>GSDSHSKQLEINVKSDKVPQKVKDLAQQQFAGYAKALDKQSNAKTGKYELGEAFKIYKFNGEEDNSYYYPVIKDGKIVYTLTLSPKNKDDLNKSKEDMNYSVKISNFIAKDLDQIKDKNSNITVLTDEKGFYFEEDGKVRLVKATPLANNIKEKESAKTVSPQLKQELKTTVTPTKVEENEAIQEDQVQYENTLKNFKIREQQFDNSWCAGFSMAALLNATKNTDTYNAHDIMRTLYPEVSEQDLPNCATFPNQMIEYGKSQGRDIHYQEGVPSYNQVDQ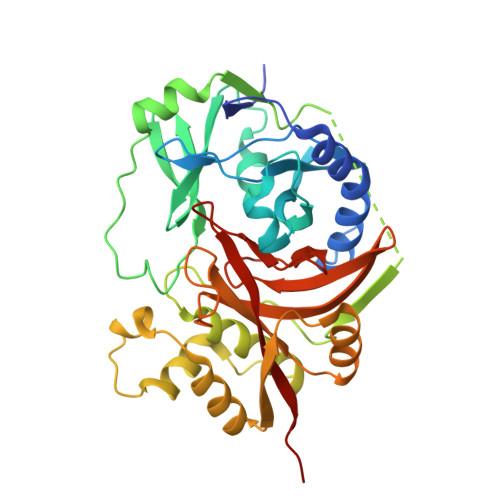LTKDNVGIMILAQSVSQNPNDPHLGHALAVVGNAKINDQEKLIYWNPWDTELSIQDADSSLLHLSFNRDYNWYGSMIGYLEVPIHRD[4x]>XGEIAKALREIAKA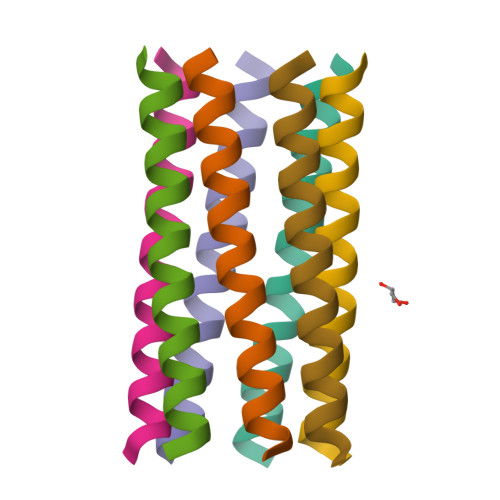LRECAWAHREIAKALRG[7x]>[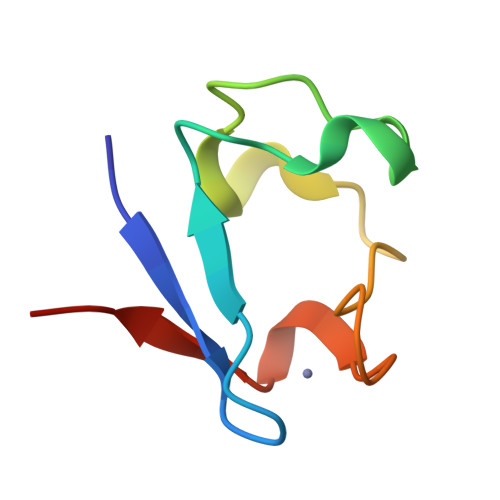8x]MKKWVCTVCGYIYDEDAGDPDNGISPGTKFEELPDDWVCPLCGVGKDQFEKLED>[2x]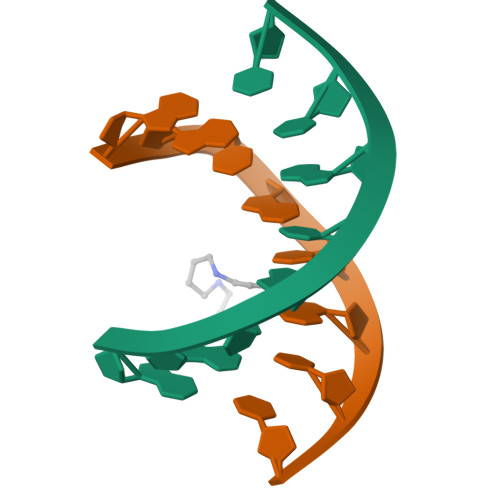GGTATACC> MSKIESALQAAQPGLSRLRGGAGGMGYRAATTQAEQPRSSLLDTIGRFAKAGADMYTAKEQRARDLADERSNEIIRKLTPEQRREALNNGTLLYQDDPYAMEALRVKTGRNAAYLVDDDVMQKIKEGVFRTREEMEEYRHSRLQEGAKVYAEQFGIDPEDVDYQRGFNGDITERNIS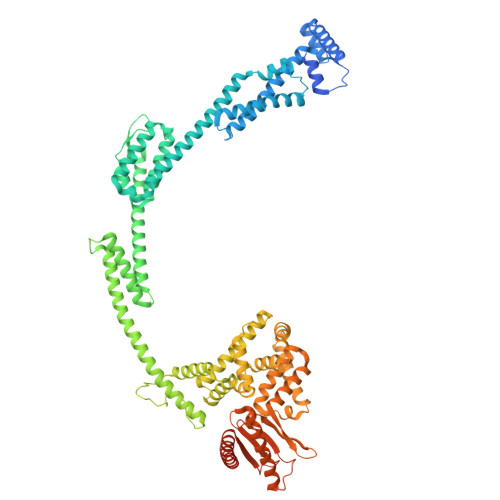LYGAHDNFLSQQAQKGAIMNSRVELNGVLQDPDMLRRPDSADFFEKYIDNGLVTGAIPSDAQATQLISQAFSDASSRAGGADFLMRVGDKKVTLNGATTTYRELIGEEQWNALMVTAQRSQFETDAKLNEQYRLKINSALNQEDPRTAWEMLQGIKAELDKVQPDEQMTPQREWLISAQEQVQNQMNAWTKAQAKALDDSMKSMNKLDVIDKQFQKRINGEWVSTDFKDMPVNENTGEFKHSDMVNYANKKLAEIDSMDIPDGAKDAMKLKYLQADSKDGAFRTAIGTMVTDAGQEWSAAVINGKLPERTPAMDALRRIRNADPQLIAALYPDQAELFLTMDMMDKQGIDPQVILDADRLTVKRSKEQRFEDDKAFESALNASKAPEIARMPASLRESARKIYDSVKYRSGNESMAMEQMTKFLKESTYTFTGDDVDGDTVGVIPKNMMQVNSDPKSWEQGRDILEEARKGIIASNPWITNKQLTMYSQGDSIYLMDTTGQVRVRYDKELLSKVWSENQKKLEEKAREKALADVNKRAPIVAATKAREAAAKRVREKRKQTPKFIYGRKE(1S)-N-[(1S)-7,7-dihydroxy-1-{4-[(1R,4S)-1,2,3,4-tetrahydro-1,4-methanonaphthalen-6-yl]-1H-imidazol-2-yl}nonyl]-6-methyl-6-azaspiro[2.5]octane-1-carboxamide 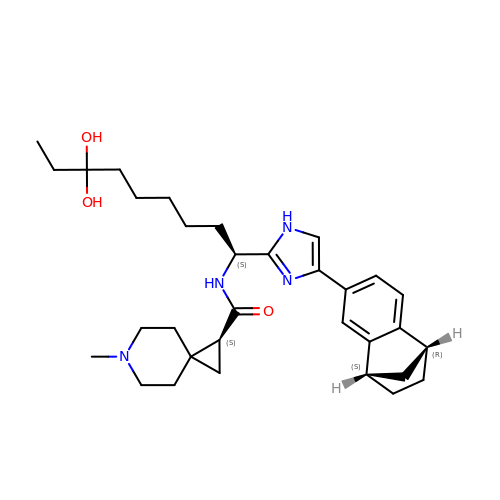| C32 H46 N4 O3 | OYAZOARGEULSKR-IMIIGWPFSA-N6-azanyl-9~{H}-purine-8-thiol | C5 H5 N5 S | 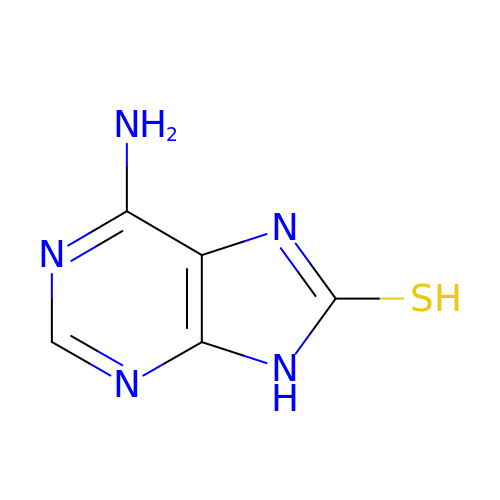BHVOFCPOXNYVCE-UHFFFAOYSA-N> EKNSKDAQKMINEMQKRNRQTNERIEEIIRTTGKENAKYLIEKIKLHDMQEGKCLYSLEAIPLEDLLNNPFNYEVDHIIPRSVSFDNSFNNKVLVKQEENSKKGNRTPFQYLSSSDSKISYETF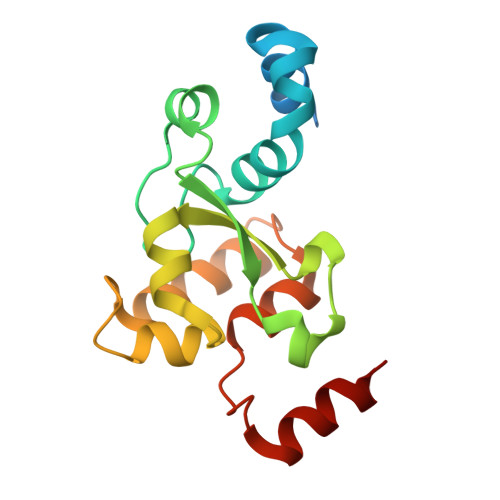KKHILNLAKGKGRISKTKKEYLLEERDINRFSVQKDFINRNL> MVISWIPPYNVPVSFENLEKSFDGYGPADGLSHIAPQFWVPDGNGGISYVTRDDYSMDYMNDDSVKVIRDWGNQYGIKTMLCIYNGEH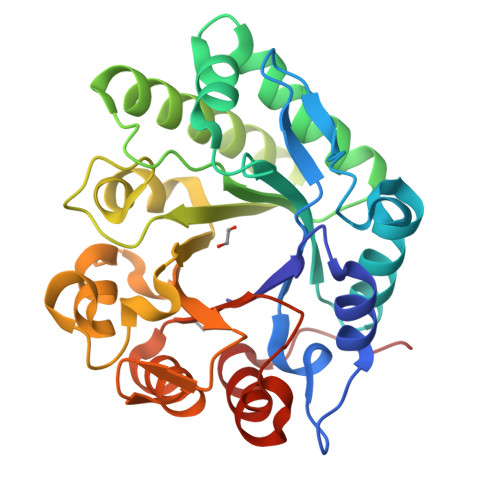GWDWSLVSTSISAANRQSFVDAIVTEMKRLNLHGVEVDLEGPNADSPTDTENFLLFMEKLSDTLSSLGKDLTIATFASREWDHIPDASHWPELLPLVDGITSMGYEETGINATGDLSYAGQKSMAAGAPEKLMLGMPDHLDSWQGSSALQQVEWAQDNGVGVALWDMQLRNEAWQRRDIWKALSEIRGPLGTTYT> MPVPESQLERWSHQGATTTAKKTHESIRAALDRYKWPKGKPEVYLQGSYKNSTNIRGDSDVDVVVQLNSVFMNNLTAEQKRRF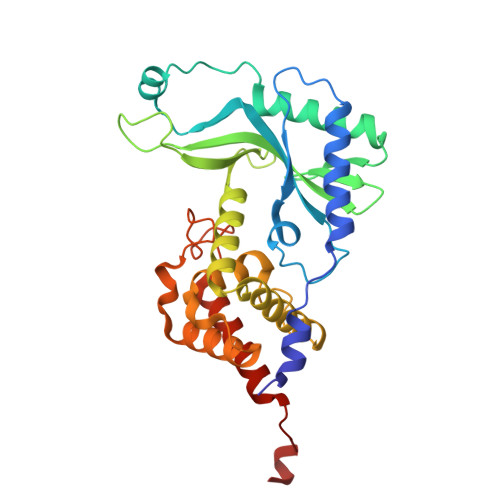GFVKSDYTWNDFYSDVERALTDYYGASKVRRGRKTLKVETTYLPADVVVCIQYRKYPPNRKSEDDYIEGMTFYVPSEDRWVVNYPKLHYENGAAKNQQTNEWYKPTIRMFKNARTYLIEQGAPQDLAPSYFLECLLYNVPDSKFGGTFKDTFCSVINWLKRADLSKFRCQNGQDDLFGEFPEQWSEEKARRFLRYMDDLWTGWGQGSHHHHHH> GTHSLKYVYTGVSRGIDFPEFTAVGMVDDGQFMYFDSNSMKAVPKTEWIRQNEGADYWDRQTQVLIGAHQVFKDSIQIVMERFNQSKGVHTWQNMYGCELNDDGTTQGFYQYAYDGEDFVSLDKNTLTWTAANPQAVITKHKWEALAVAEQNKGYLENTCIEWLKKYVAYGKDTLERKVSPQVSLLQKDPSSPVTCHATGFYPSGVTITWQKNGQDHDEDVDLGELLPNEDGSFQ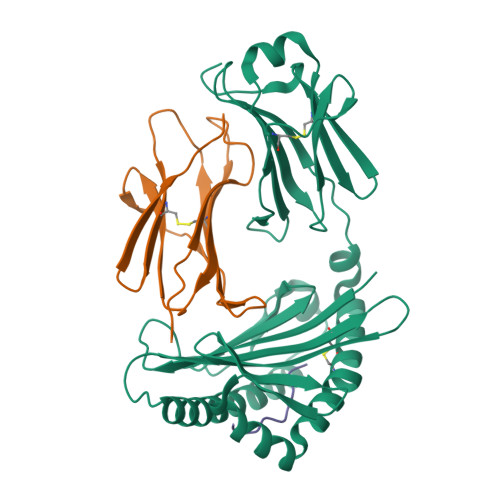RMSTLNVGPDEWKNNRFSCVVEHQDKTIRKTEDDIITNFD;> MKVSSPKIQVYSHYPGEYGKENTLICYVSNFHPPDISIELLKNGKVIADAQQTDLAFEKGWQFHLTKSVSFKPEKSDEYSCRVKHMSDNKTIVWESNM;> FANFCLMMI> MAFPAGFGWAAATAAYQVEGGWDADGKGPCVWDTFTHQGGERVFKNQTGDVACGSYTLWEEDLKCIKQLGLTHYRFSLSWSRLLPDGTTGFINQKGIDYYNKIIDDLLKNGVTPIVTLYHFDLPQTLEDQGGWLSEAIIESFDKYAQFCFSTFGDRVKQWITINEANVLSVMSYDLGMFPPGIPHFGTGGYQAAHNLIKAHARSWHSYDSLFRKKQKGMVSLSLFAVWLEPADPNSVSDQEAAKRAITFHLDLFAKPIFIDGDYPEVVKSQIASMSQKQGYP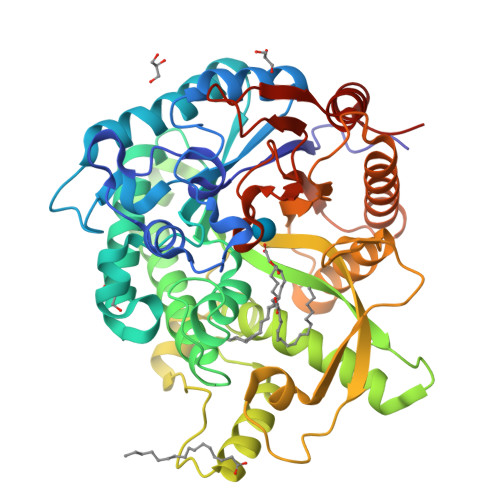SSRLPEFTEEEKKMIKGTADFFAVQYYTTRLIKYQENKKGELGILQDAEIEFFPDPSWKNVDWIYVVPWGVCKLLKYIKDTYNNPVIYITENGFPQSDPAPLDDTQRWEYFRQTFQELFKAIQLDKVNLQVYCAWSLLDNFEWNQGYSSRFGLFHVDFEDPARPRVPYTSAKEYAKIIRNNGLEAHL N-{4-[3-(2-amino-4-oxo-3,4-dihydrothieno[2,3-d]pyrimidin-6-yl)propyl]thiophene-2-carbonyl}-L-glutamic acid | C19 H20 N4 O6 S2 | 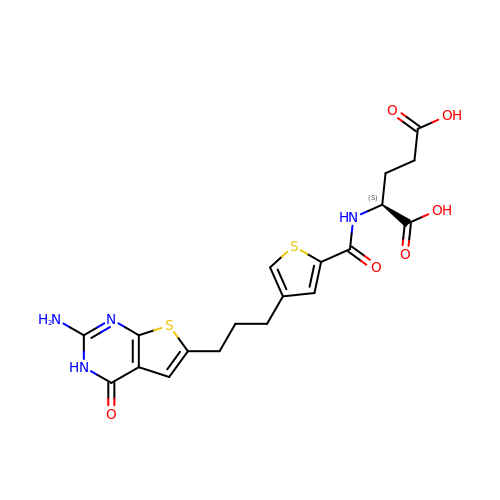QXWUFUZJYLBZQF-LBPRGKRZSA-N>[4x]IAFDALREPDRESSAPPDDVQLVPGARIANGRYRLLIFHGGVPPLQFWQALDTALDRQVALTFVDPQGVLPDDVLQETLSRTLRLSRIDKPGVARVLDVVHTRAGGLVVAEWIRGGSLQEVADTSPSPVGAIRAMQSLAAAADAAHRAGVALSIDHPSRVRVSIDGDVVLAYPATMPDANPQDDIRGIGASLYALLVNRWP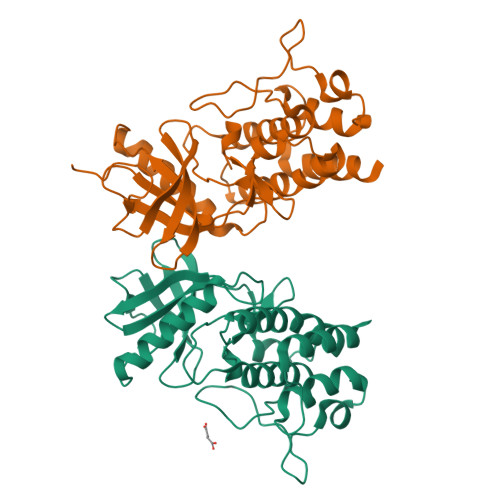LPEAGVRSGLAPAERDTAGQPIEPADIDRDIPFQISAVAARSVQGDGGIRSASTLLNLMQQATAVADRTEVLGPIDEAPVSAAPR> SSLPVPYKLPVSLSVGSCVIIKGTPIHSFINDPQLQVDFYTDMDEDSDIAFHFNVHFGNHVVMNRREFGIWMLEETTDYVPFEDGKQFELCIYVHYNEYEIKVNGIRIYGFVHRIPPSFVKMVQVSRDISLTSVCVCN

Galectin (Gal) is a lectin that binds to β-galactosides. Because the primary and tertiary structures of Gal-13 are highly conserved among all galectins, it had been named galectin-13. However, our crystallographic and biochemical experiments (solid phase experiment, hemagglutination assay, and biolayer interferometry) proved that wild-type Gal-13 could not bind lactose or a rhamnogalacturonan Ι domain (RG-I-4) from Ginseng Pectin. Primary structure alignment showed that a highly conserved histidine residue was modified to arginine (Arg53) in the ligand binding site of wild-type Gal-13, which may be why Gal-13 could not bind lactose.

Tris has three hydroxyl groups and binds in a triangular shape. Aside from R53H, the double mutant R53HR55N also could co-crystallize with Tris, but not lactose. The Tris molecule in R53HR55N occupies a different position compared with Tris in R53H. It seems that Arg55 plays a role in stabilizing Tris in R53H. In contrast, Asn55 could not stabilize Tris, and its hydroxyl group points up in direction. Here, we found two Gal-13 variants (R53H and R53HR55N) that could co-crystallize with Tris, that also has three hydroxyl groups and shows a triangular shape when bound in the ligand binding site. However, the hydroxyl groups from Tris could not be merged with the oxygen atoms of lactose.> MRHPLQCHW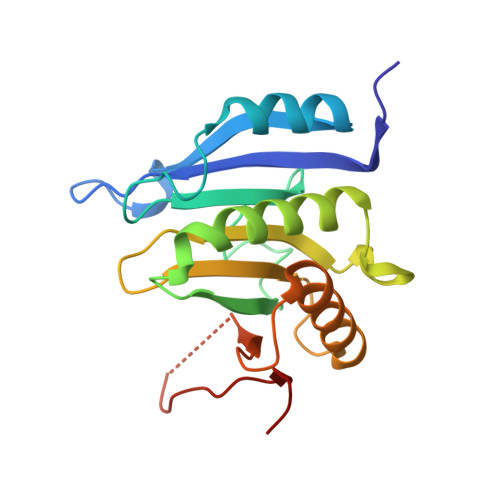ALWYLKADRSKDWEDCLKQVAVFDTVEDFWSLYNHIQAASGLTWGSDYYLFKEGIKPMWEDENNVKGGRWLVVVDKQKRAQLLDHYWLELLMAIIGEQFEDNGEYICGAVVNVRQKGDKVSLWTRDSLKDDVNLRIGQILKAKLEIPDTEPIRYEVHKDSSVRTGSMVKPRIVIPSKDNR> MRGSHHHHHHGSMPVAGSELPRRPLPPAAQERDAEPRPPHGELQYLGQIQHILRCGVRADDRTGTGTLSVFGMQARYSLRDEFPLLTTKRVFWKGVLEELLWFIKGSTNAKELSSKGVKIWDANGSRDFLDSLG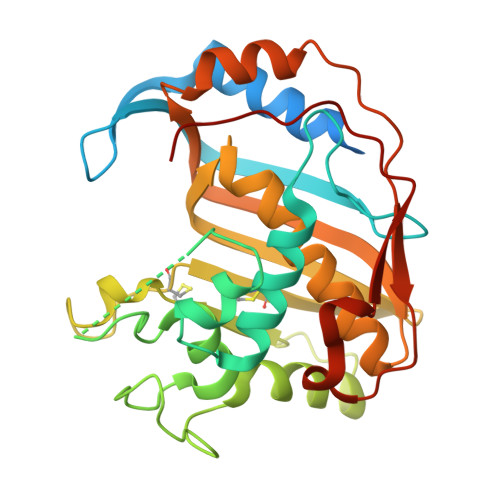FSTREEGDLGPVYGFQWRHFGAEYRDMESDYSGQGVDQLQRVIDTIKTNPDDRRIIMCAWNPRDLPLMALPPCHALCQFYVVNSELSCQLYQRSGDMGLGVPFNIASYALLTYMIAHITGLKPGDFIHTLGDAHIYLNHIEPLKIQLQREPRPFPKLRILRKVEKIDDFKAEDFQIEGYNPHPTIKMEMAV methyl 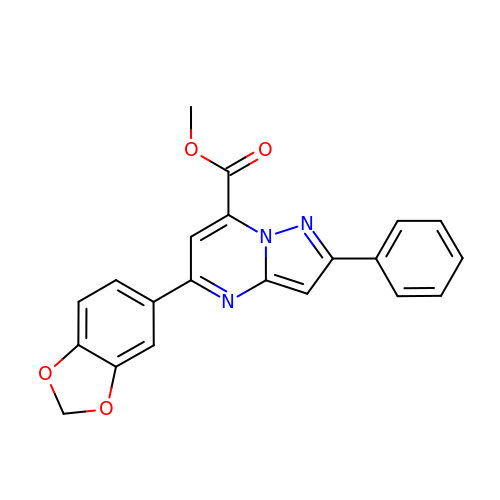5-(1,3-benzodioxol-5-yl)-2-phenyl-pyrazolo[1,5-a]pyrimidine-7-carboxylate | C21 H15 N3 O4 | DCSWTUKGGUNNLU-UHFFFAOYSA-N(1E,4E,8E)-2,6,6,9-Tetramethyl-1,4-8-cycloundecatriene | C15 H24 | 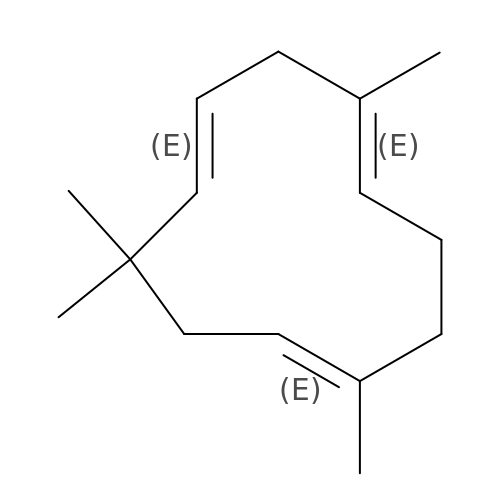FAMPSKZZVDUYOS-HRGUGZIWSA-N> MGSSHHHHHHSSGLVPRGSHMQEQTAKEDVADSATSVGAIVSIEKAEKNFVITYASGKKAQISILNDHLFRYHLDPTGKFEEYPTPNDPKHVAKITAKTMADYGTQAFEQTNVTDSGNQFILENNGLKIIFEKESALMKVLDKKKNQVILEETAPLSFKNDK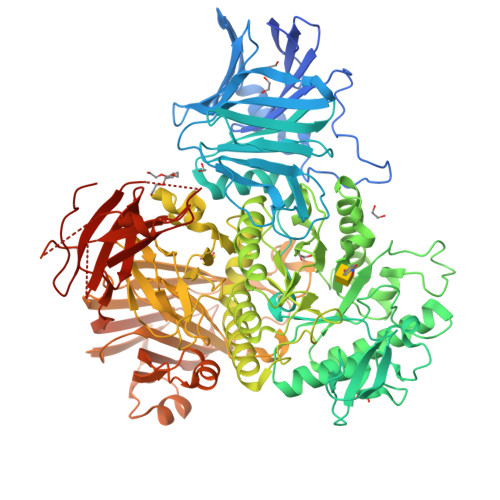ATQTLKQSSQENYFGGGTQNGRFTHKGTAIQIVNTNNWVDGGVASPNPFYWSTAGYGVVRNTWKPGNYDFGSHDPQTTTTTHEGTDFDAFYFFNDSSAGILKDYYELTGKPALMPEYGFYEAHLNAYNRDYWVKVAEGTAGAVKFEDGNFYKEYQPGDLGNLNGTLESLNGEKENYQFSARAVIDRYKKNDMPLGWFLPNDGYGAGYGQTDSLDGDVQNLKEFTDYAQANGVEVGLWTQSNLHPADPKNPKKGERDIAKEVSVAGVKALKTAVAWVGYGYSFGLNGVEDAANVFVKETDGAVRPMIVSLDGWAGTQRHAGIWTGDQTGGQWEYIRFHIPTYIGTSLSGQPNVGSDMDGIFGGKNKEVNIRDFQWKTFTPVQLNMDGWGSNPKTPFAFDQEATDLNRAYLKLKSMMMPYNYSIAKESVDGLPMVRAMALEFPNEGTAYTKDSQYQYMWGPNLLVAPIYNGNQDEAGNSIRDGIYLPDEKQVWVDLFTGEKYQGGRVLNGVKTPLWKVPVFVKDGSIIPMTNPNNNPKEIQRDQRSFLIYPNGATSFNMYEDDGISTSYEAGQSATTKINSQGPKSNEKGDLTVTIEPTKGSYKDFVDERSTTLDLLASEAPESVTAMVGGTEVTLKQAANKEEFLAGTNLYYFDKEFQVNQYLSEASGEKLNQSALSVKLAKQSVTAKDVQITVKGFINKGTVDGGNTTVDDQLTIPANIAINEEKTTPSSLTLQWDQVTEATSYEVERDGTVFGNIQTNTATFDGFSFLSEHTFRVRAVGKNGVSEWSEPIKGKTQDDPYK>MKVLALRHSVAQVYADTQIYTHDDTKDSYENAFLISNLTTHNILYFNYSARTLEILNKSGIAAIEIQSLEELFTLIRCNFTYDYENNVVYLHDYSYYTNNEIRTDQHWITKTNIEEYLLPGWKLTYVGYNGNDTRGHYNFSFTCQNAATDDDIIIEYIYSEALDFQNFMLRKIKERMTTSLPIARLSNRVFRDKLFPLLVKKHKRVVNVGPRNESMFTFLNFPSIRQFSNGPYLVKNTIKLKQERWLGKRVSQFDIGQYKNMLNVITTIYHYYNLYQEKPIIYMVGSAPSYWIYDVRQYSDFLFETWDPLDTPYSSIHHKELFFAKDIGKLKDNSILYIDIRTDRGNADWKEWRKVVELQTISNLNLAYQYLATGKSKVCCVKLTAMDLELPVSAKLLHHPTTEIRSEFYLLLDIWDVNNIKRFIPKGALYSFINNVITDNVFIQSPFKIRTSVSDYIVALYALSNDFNNREDIINLINNQKQSLITVRINNTFKDEPKVGFKSIYDWTFLPTDFETTNAIVTSYDGCLGIFGLSISLASKPTGNNHLFILNGTDKYYKLDQFANHTGISRRSHQVRFSESATSYSGYIFRDLSNSNFNLIGTNV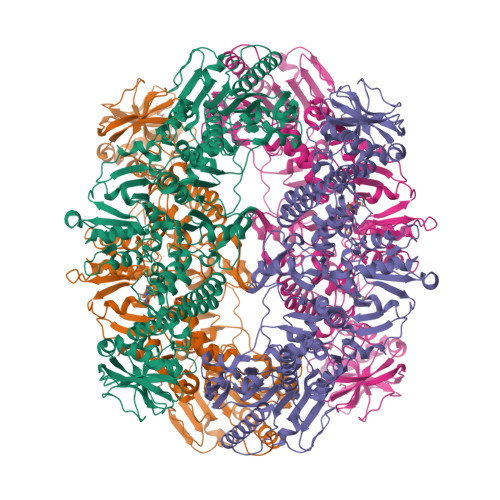ENSVSGHVYNALIYYRYNYSFDLKRWIYLHSVEKANIEGGKYYEHAPIELIYACKSAKEFASLQDDLTVLRYANEIENYINKVYSITYADDPNYFIGIKFNNIPYIYDVKVPHLTFGVLYISDNMIPDVVKIMKSMKQELFGMDVTTSYTYMLSDGVYVANVSGVLATYFKMYNLFYKNQITFGQSRMFIPHITLSFSNNKTVRIETTKLRIKSIYLRKIRGDTVFDMPE[3x]>MNSKMEFTDRAKKALEDAMALAEQYQHLQLQPVHLAVALLDPTPDPSKDQSIAPGTTSTLFRQVVERAHGDAQAFDRALKKKLVRLPSQDPPPDQVSMSAGCSNVLRKANELQKVQKDSYIAVDHLIAALAEDHAIQEALKEANIPKPKLIQDAIQAIRGNKRVDSRNADTEQENENLSKFCIDMTAMAREGKIDPVIGREEEIRRVIRILSRRTKNNPVLIGEPGVGKTTIVEGLAQRIVNADVPDNLAACKLLSLDVGALVAGSKYRGEFEERMKGVLKEIQESKETIILFVDAIHLLMGAGSSGEGGMDAANLLKPMLARGQLHCIGATTLAEYRKYIEKDAAFERRFQQVLVKEPSISETISILRG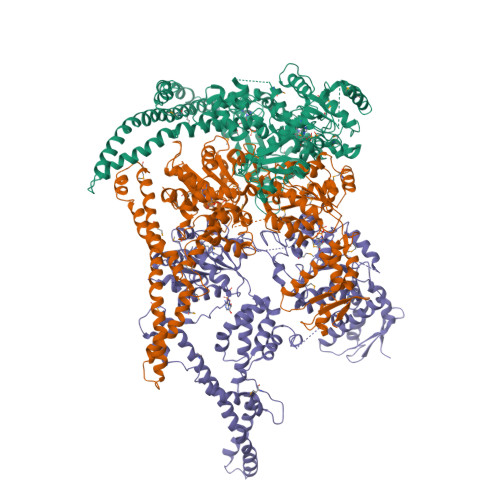LKEKYEVHHGVNIADAAIVAAANLAARYLTSRRLPDSAVDLIDEAAAAVRVARESQPEIIDSLERRLRQLKIEIHALSREKDEASKARLAQAKQDAQNVEEELRPLREKYERERQRGKAIQEAKMKLEALRVKAEDASRMGDHSRAADLQYYAIPEQEAIIKRLEAEKAAADAALNANGADVGGSMITDVVGPDQINEIVARWTGIPVTRLKTSEKEKLLHMEQALSKIVVGQKEAVQSVSNAIRLQRSGLSNPNQPPSFLFCGPSGTGKTLLTKALAEFLFDDPKSMIRFDMSEYQERHSLSRMIGAPPGYVGHDAGGQLTEALRRRPFSILLFDAVEKAAKEVLTVLLQLMDDGRITDGQGRVVDAKNCIVVMTSNLGAEYLSRANNGKDGKIDPTTRELVMNTLRNYFLPEFLNRISSVVIFNRLTRREIRKIVDLRIAEIQKRLTDNDRNVIIKVSEEAKDKLGAQGYSPVYGARPLQRLLEKEVLNRLAILILRGQIREGEVAHVELVDGKVQVLPNHPDSEPEDVDVDMDSDDAVDEVAPDSMDEDIYND[3x]>[2x]AMAIPAFHPGELNVYSAPGDVADVSRALRLTGRRVMLVPTMGALHEGHLALVRAAKRVPGSVVVVSIFVNPMQFGAGGDLDAYPRTPDDDLAQLRAEGVEIAFTPTTAAMYPDGLRTTVQPGPLAAELEGGPRPTHFAGVLTVVLKLLQIVRPDRVFFGEKDYQQLVLIRQLVADFNLDVA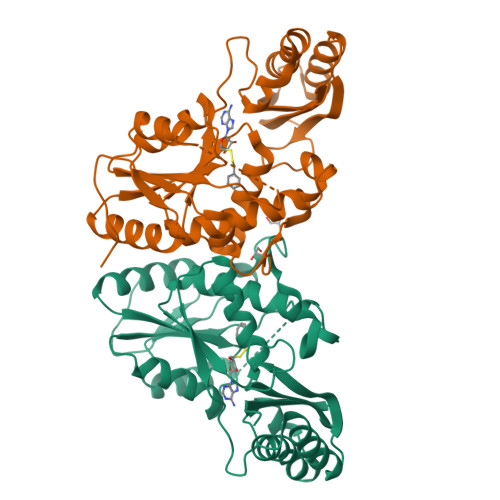VVGVPTVREADGLAMSSRNRYLDPAQRAAAVALSAALTAAAHAATAGAQAALDAARAVLDAAPGVAVDYLELRDIGLGPMPLNGSGRLLVAARLGTTRLLDNIAIEIGTFAGTDRPDGYR>[4x]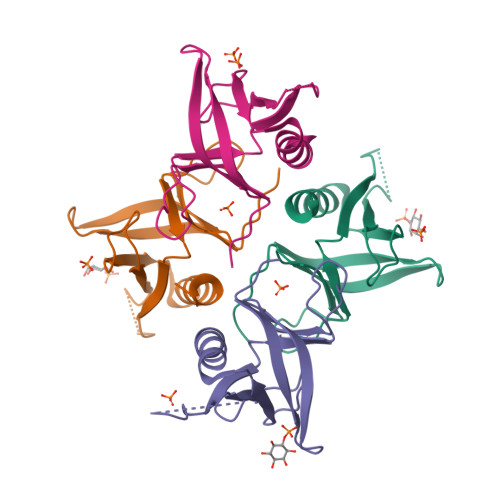DHPFTEIKSGFLERRSKFLKSYSKGYYVLTPNFLHEFKTADRKKDLVPVMSLALSECTVTEHSRKNSTSSPNSTGSDAKFVLHAKQNGIIRRGHNWVFKADSYESMMSWFDNLKILTSTS>MDYKDDDDKGRLRRRQEIIDHEEEESNDDVSSRRGKLSLAETFRWLDSSEHRRIETDGHNDYKYIIHPKNRWYKAWEMFILVWAIYSSLFTPMEFGFFRGLPERLFVLDIVGQIAFLVDIVLQFFVAYRDTQTYRTVYKPTRIAFRYLKSHFLMDFIGCFPWDLIYKASGKHELVRYLLWIRLFRVRKVVEFFQRLEKDTRINYLFTRILKLLFVEVYCTHTAACIFYYLATTLPPENEGYTWIGSLKLGDYSYENFREIDLWKRYTTALYFAIVTMATVGYGDIHAVNLREMIFVMIYVSFDMVLGAYLIGNITALIVKGSNTERFRDKMNDLISFMNRKKLGRDLRSQITGHVRLQYDSHYTDTVMLQDIPASIRAKIAQLLYLPYIKKVPLFKGCSTEFINQIVIRLHEEYFLPGEVITEQGNVVDHLYFVCEGLLEALVTKTDGSEESVTLLGPHTSFGDISIICNISQPFTVRVCELCHLLRLDKQSFSNILEIYFHDGRTILNNIMEEKESNDRIKKLESDIVIHIGKQEAELALKVNSAAFQGDFYQLKSLIRSGADPNKTDYDGRSPLHLAACRGYEDITLFLIQEGVDVNLKDKFGHTPLFEAVKAGQEGVIGLLVKEGASFNLEDSGNFLCTTVAKGDSDFLKRLLSSGMNPNSEDYDHRTPLHVAASEGLFLMAKMLVEAGASVISKDRWGNSPLDEARLCGNKKLIKLLEDVKNAQSSIYPSSLRELQEERIERRKCTVF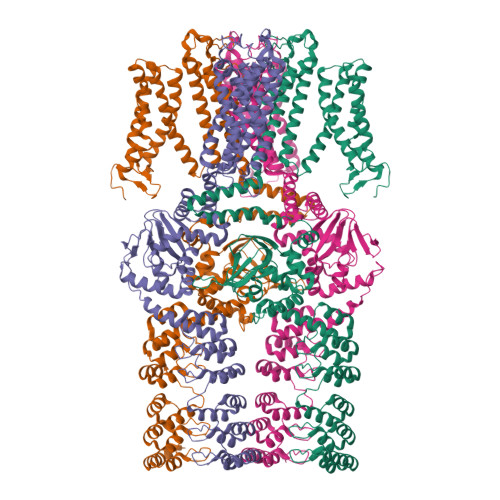PFHPQEAKEERSRKHGVVVWIPSNLEKLIVTAAKELGLSDGASFVLLSEDQGRITDIDMISDGHKLYMISDTTDQTHHHHHH[4x]GAMMA-ARSONO-BETA, 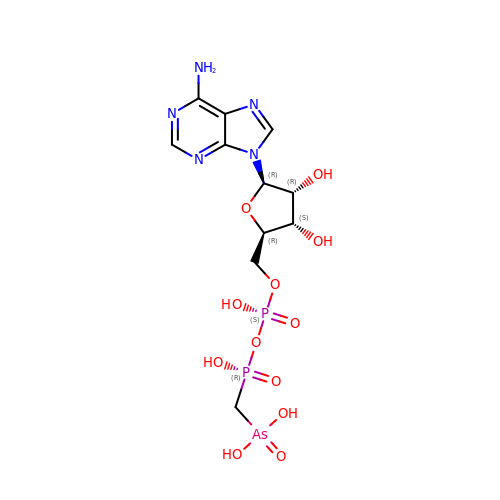GAMMA-METHYLENEADENOSINE-5'-DIPHOSPHATE | C11 H18 As N5 O12 P2 | KHQOAQLQNLUEQN-IOSLPCCCSA-N> LGLDCDEHSSESRCCRYPLTVDFEAFGWDWIIAPKRYKANYCSGQCEYMFMQKYPHTHLVQQANPRGSAGPCCTPTKMSPINMLYFNDKQQIIYGKIPGMVVDRCGCS;> TRECIYYNANWELERTNQSGLERCEGEQDKRLHCYASWRNSSGTIELVKKGCWLDDFNCYDRQECVATEENPQVYFCCCEGNFCNERFTHLPEPG;> ALQCFCHLCTKDNFTCVTDGLCFVSVTETTDKVIHNSMCIA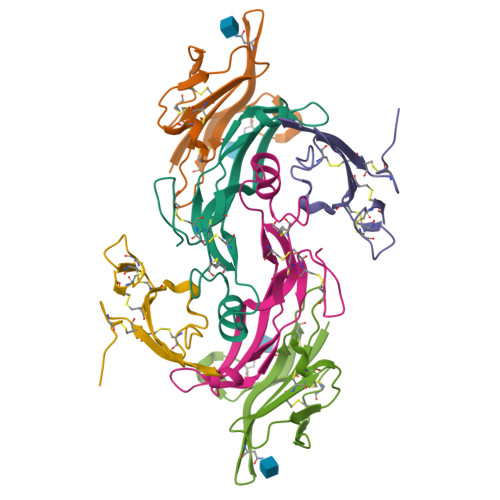EIDLIPRDRPFVCAPSSKTGSVTTTYCCNQDHCNKIELP> EEYSAM;> AKCVSYGVAQIKAPALHSQGYTGSNVKVAILDTGIDSSHPDLNVAGGASFVPSETNPFQDNSSGGTHIAGTVLAVAPSASLYAVKVLGADGKGQASWIINGIEWAIANNMDVINMSLGSPSGSAAVKAAVDKAVAS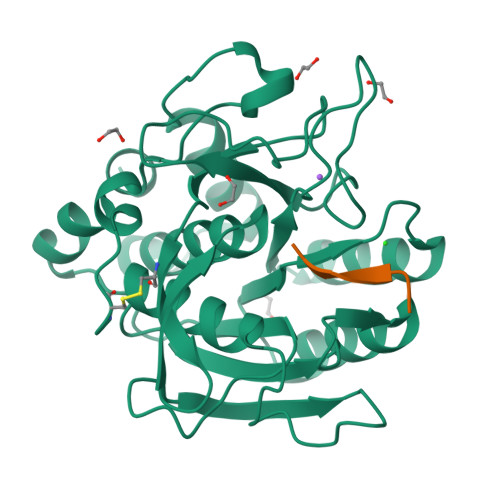GVVVVAAAGNSGTSGSSSTVTYPAKYPSVIAVGAVDSSNQRAPFSSVGPELDVMAPGVSICSTLPGGKYGALSGTSMASPHVAGAAALILSKHPNWTNTQVRSSLENTATKLGDSFYYGKGLINVEAAAQ3-[1-(4-chlorobenzyl)-5-(2-fluoro-2'-methylbiphenyl-4-yl)-3-methyl-1H-indol-2-yl]-2,2-dimethylpropanoic acid | C34 H31 Cl F N O2 | 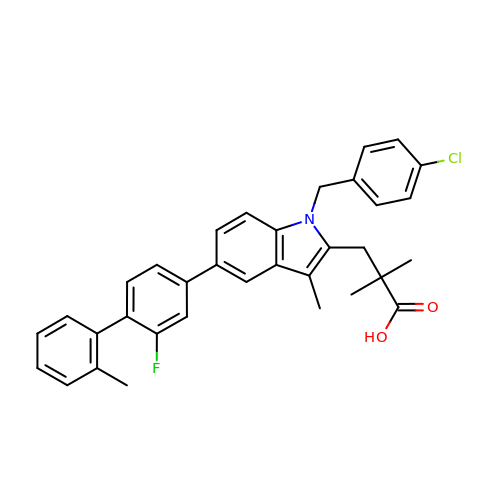IYCJVTFMIQICDJ-UHFFFAOYSA-N Glutathione, the tri-peptide γ-L-glutamyl-cysteinyl-glycine, is the main low molecular weight thiol antioxidant in both plant and animal cells, often present at millimolar concentrations in vivo. It is synthesised in a two-step, ATP-dependent, process: glutamate-cysteine ligase (GCL) catalyses the formation of γ-glutamylcysteine (γ-EC) from glutamate and cysteine, followed by the addition of glycine by glutathione synthetase (GS) to form glutathione. Cyst nematodes have exploited a series of gene gain events to redeploy glutathione synthetase-like enzymes during parasitism, within the syncytial feeding cell formed in the host root. The most recent expansion has been coupled with a diversification of structure and biochemical function that has given rise to enzymes that are introduced into the host cell, and likely possess novel substrate specificities.

For comparison, the only GS gene in the corresponding plant host of G. pallida (Solanum tuberosum, St-gss1), was similarly expressed and its product purified. Using this approach, the maximum rate of the host GS (St-GSS1) phosphate release was 7532 (±1358) umol/mg/min, consistent with a previous report for Arabidopsis GS of ~7500 umol/mg/min, demonstrating the suitability of the assay. St-GSS1, Clade 1 Gpa-GSS1, and Clade 2 Gpa-GSS5 all exhibited a strong preference for glycine, and a high affinity for γ-EC. Residues in the ATP binding pocket of St-GSS1 are highly conserved in sequence and position in the Gpa-GSS22 structure (13/15 residues), and similarly conserved in sequence across G. pallida Clade 3 (structure guided alignment, ~12/15, n = 24). The position of γ-EC in St-GSS1 is coordinated at both the glutamate and the cysteine residue. Two of the three residues that coordinate the cysteine interact with the C-alpha backbone. Corresponding residues in all G. pallida GS-like effectors are not conserved in sequence but are preferentially small and uncharged, while the third residue, arginine, is 100% conserved: consistent with permitting interactions with a cysteine residue. However, the glutamate of the di-peptide is exclusively coordinated by interactions with charged side chains of residues in the binding pocket (R, E, 2xQ, N, and Y). All six of these positions are substituted in Gpa-GSS22 and Gpa-GSS30, thus suggesting that the lack of canonical activity is because γ-EC is not accepted despite the potential for cysteine to be accommodated.

>MQTQVEDSAKPIVDPHDIDPKLVQKLANDALVWCSLRGLLVGDRNSERSGTVPGVDMVHAPVALIPMSFPESHWKQACEVAPIFNELVDRVSQDGEFLQQSLSRTRKVDPFTSRLLEIHSKMLEINKIEEIRLGLHRSDYMLDEQTKLLLQIELNTISSSFPGLSCLVSELHRSLLQQYREDIASDPNRIPANNAVNQFAEALAKAWNEYGDPRAVIMFAVQAEERNMYDQHWLSASLRERHQVTTIRKTLAEIDALGELQQDGTLVVDGQAVAVIYFRAGYAPSDYNSESEWKARLLMEQSRAVKCPSISYHLAGSKKIQQELAKPNVLERFLENKDDIAKLRKCFAGLWSLDESDIVKDAIDRPELYVMKPQREGGGNNIYGEDVRDALLKLQKEGTGSDAAYILMQRIFPKISHSILMREGISHKEQTISELGIYGTYLRNKTEVVINQQAGYLMRTKVSSSNEGGVAAGFAVLDSIYLV[6x]>MTLSIIVAHDKQRVIGYQNQLPWHLPNDLKHIKQLTTGNTLVMARKTFESIGKPLPNRRNVVLTNQASFHHEGVDVINSLDEIKELSGHVFIFGGQTLYEAMIDQVDDMYITVIDGKFQGDTFFPPYTFEDWEVESSVEGQLDEKNTIPHTFLHL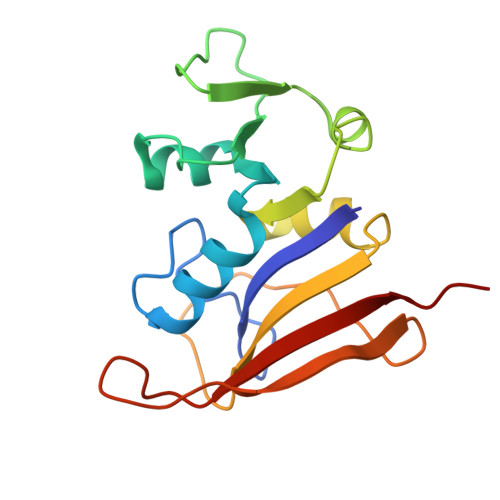VRRKGK[2x]>ERFKVVCYYTNWAWYRPDNGKYTPGDINPELCTHIIYAFAVLDKEELVIKSHDIWLDVENKFYEKVTALKSHGVKVLLGLGGWDDSAGDKYSRLVNNVSARRKFVVHAVDFLEQYGFDGLDLDWEYPKCWQVECEKGPDSDKQGFADLVKELRKAFNRRGMLLSAAVSASKRVIDYAYNVPALSMNLDWISLMTYDYHGQWDKKTGHVAPMYVHDKDTDNTFNVNFTVNYWINKGADRKKLVVGVPFYGQSFSVVEGAGTGLGAPTYAGGEAGDETRARGFLSFYEICERVKVKGWKVHRDPGGRIGPYATHDDQWVSFDDDFMARHKAEYVRAMELGGSMAWSLDLDDFTGKYCGCGKAPLLTTINHVLRGKEAPPPCI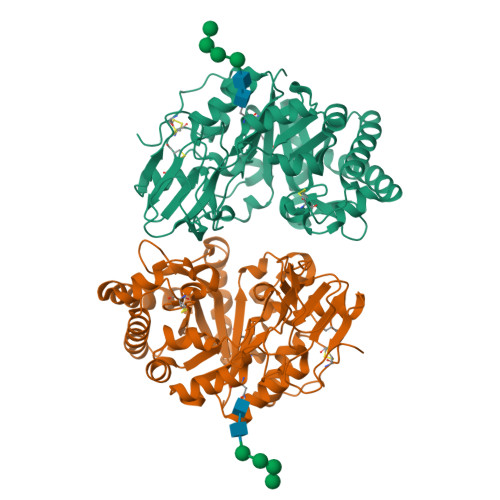LHE[2x]> GPAAVASSSKVVAGTEFPISLGSKISTVVKRPKQKKRSKKAKEDEEEILVIEGIEFDRDVAVKFDVYVNDVDDLPSGPDKTEFAGSFVSVPH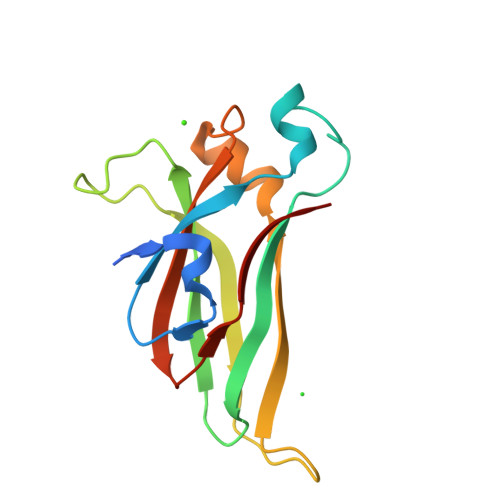SHKHKKKMNTILRLGLTDLLEEIEAEDDDSVVVTLVPKFGAVKIGGIKIEFAS>SEREEELKRLKKEQEKIREEIEEVKKEIEESKKRPQSESQKNFILSLQLFISMLRLKLLWSRALALQLQRERLTDTDEVDRRREQELKRLKKELEKLREETEEVKKEIEESKKRPQSESLKNIILINQLLILVIRSEYLIIRNLISQLQAQTNPNNTRLKQEQKRSKKEQEKIREELEEVKKEIEESKKRPQSESAKNFILMAQSLISLIRLLALITRALNLQLQARRDGPNEELEQELKRLKKEVEKIREEQEEVNKEIEESKKRPQSESLKNFILLAQ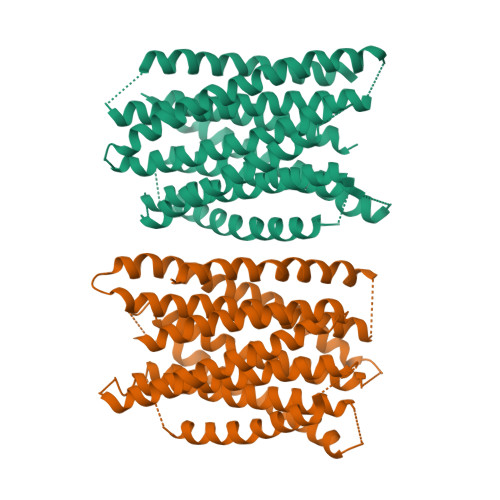LISSMVRLWELIIRILQLQLQKRKGINEDELREELKRLKKETEKIREETEEVKKEIEESKKKASQTKEIILMLQLEIAWIRSLLSIIRLLKLQLEQIDK[2x]> MLYEDPPDQKTSPSGKPATLKICSWNVDGLRAWIKKKGLDWVKEEAPDILCLQETKCSENKLPAELQELPGLSHQYW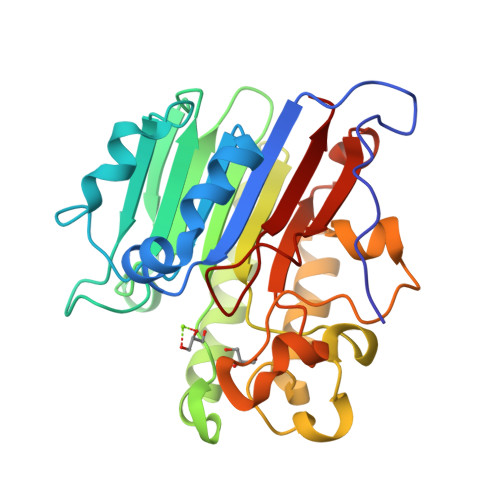SAPSDKEGYSGVGLLSRQAPLKVSYGIGDEEHDQEGRVIVAEFDSFVLVTAYVPNAGRGLVRLEYRQRWDEAFRKFLKGLASRKPLVLCGDLNVAHEEIDLRNPKGNKKNAGFTPQERQGFGELLQAVPLADSFRHLYPNTPYAYTFWTYMMNARSKNVGWRLDYFLLSHSLLPALCDSKIRSKALGSDHCPITLYLAL> MAAPGSARRPLLLLLLLLLLGLMHCASAAMFMVKNGNGTACIMANFSAAFSVNYDTKSGPKNMTFDLPSDATVVLNRSSCGKENTSDPSLVIAFGRGHTLTLNFTRNATRYSVQLMSFVYNLSDTHLFPNASSKEIKTVESITDIRADIDKKYRCVSGTQVHMNNVTVTLHDATIQAYLSNSSFSRGET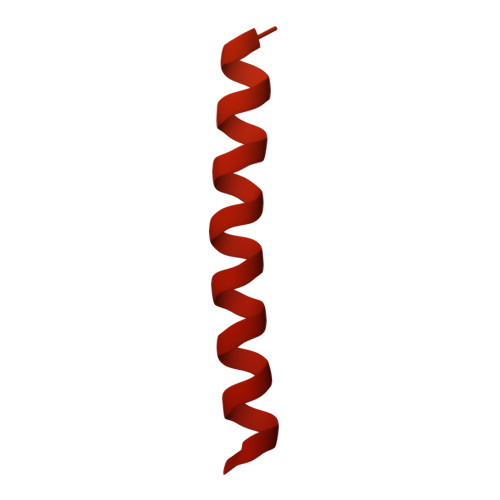RCEQDRPSPTTAPPAPPSPSPSPVPKSPSVDKYNVSGTNGTCLLASMGLQLNLTYERKDNTTVTRLLNINPNKTSASGSCGAHLVTLELHSEGTTVLLFQFGMNASSSRFFLQGIQLNTILPDARDPAFKAANGSLRALQATVGNSYKCNAEEHVRVTKAFSVNIFKVWVQAFKVEGGQFGSVEECLLDENSMLIPIAVGGALAGLVLIVLIAYLVGRKRSHAGYQTI>[2x]GSHERAIKYLNQDYETLRNECLEAGALFQDPSFPALPSSLGFKELGPYSSKTRGIEWKRPTEICADPQFIIGGATRTDICQGALGDSWLLAAIASLTLNEEILARVVPLDQSFQENYAGIFHFQFWQYGEWVEVVVDDRLPTKDGELLFVHSAEGSEFWSALL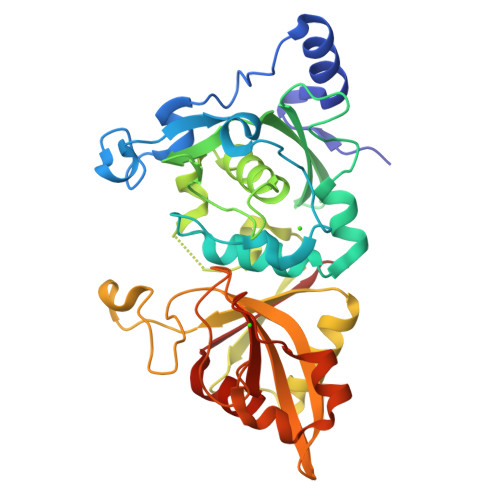EKAYAKINGCYEALSGGATTEGFEDFTGGIAEWYELRKPPPNLFKIIQKALEKGSLLGCSIDITSAADSEAVTYQKLVKGHAYSVTGAEEVESSGSLQKLIRIRNPWGQVEWTGKWNDNCPSWNTVDPEVRANLTERQEDGEFWMSFSDFLRHYSRLEICNLTPD>MELKHLPKYKHITEHAETYANIDAGSLELFLSLFDISKKMNHVMEHYFAGRGL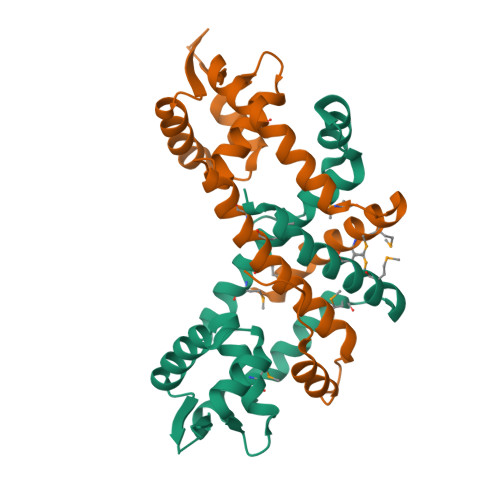SEGKFKILMLLFDAKDHRLSPTELAKRSNVTKATITGLLDGLARDGFVSRRHHTEDKRKISIELTTEGKARLEQFLPGHFSKISAVMENYSDEEKDMFVKMLGDLFERLSVFKD[2x]> MKIDTTVTEVKENGKTYLRLLKGNEQLKAVSDKAVAGVNL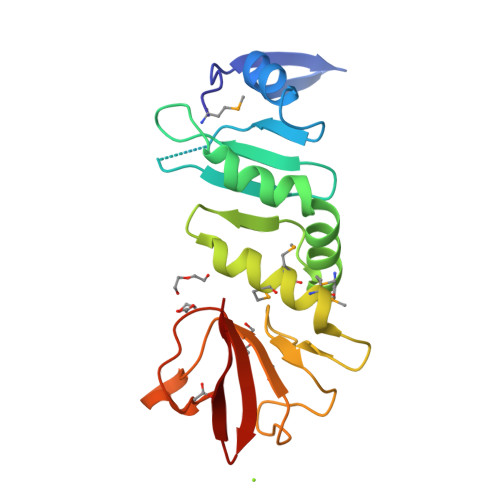FPGAKIGSFLVRQDNIVVFPDNKGEFDLDFFNLLNDNFETLVEYAKMADCLDIAFDINEKSYFNMIMWLMKNIDENWSQSPYGESFYSSKDIDWGYKPEGSLRVSDHWNFGQDGEHCPTAEPVDGWAVCKFENGKYHLIKKF>[3x]MNTISILSTTDLPAAWQIEQRAHAFPWSEKTFFGNQGERYLNLKLTADDRMAAFAITQVVLDEATLFNIAVD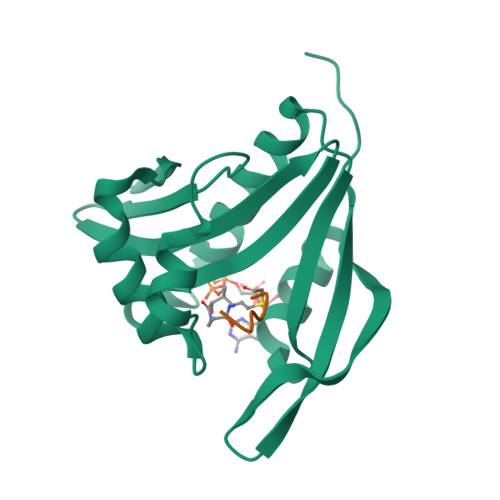PDFQRRGLGRMLLEHLIDELETRGVVTLWLEVRASNAAAIALYESLGFNEATIRRNYYPTAQGHEDAIIMALPISMKLHHHHHHHHHH;>XARYFRR[3x]>XGEIAKALREIAK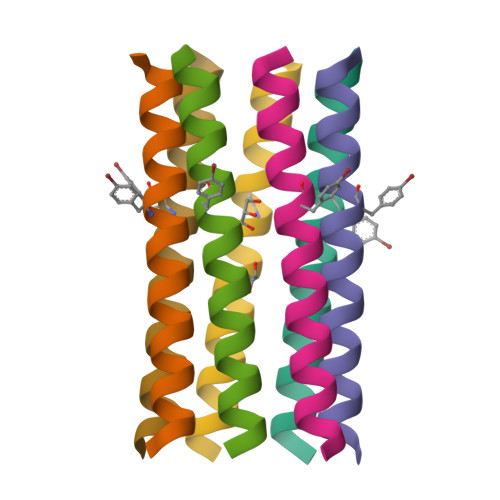ALREKAYALREIAKALRG[7x]5’-Cytosolic nucleotidase IIIB (cN-IIIB) is one of the most recently discovered 5’-nucleotidases and has several unique structural and functional features. However, one of the most preferred cN-IIIB substrates is m7GMP, for which the activity of dephosphorylation is characterized by one order of magnitude lower KM constant compared to the other preferred substrates, whereas kcat/KM is comparable. The crystal structure of cN-IIIB consists of two distinct domains: the globular core domain (residues 1–51, 132–182, and 215–300) and the smaller CAP domain (52–131 and 183–214). The core domain is a haloacid dehalogenase domain (HAD).

To date, these are the first coordinates obtained for human cytosolic nucleotidase IIIB. The second domain mainly consists of a bundle of helices that are responsible for recognizing the ligand. The C-terminal part of the protein (residues 291–300) and one of a loop connecting domains (residues 211–220) were not defined in the electron density map, and thus are most likely disordered. In all three crystal structures, the magnesium ion was octahedrally coordinated by the carboxyl side chains of catalytic moieties of Asp 41 and Asp 230 and the backbone carbonyl of Asp 43 and by three water molecules. The differences between solved structures: the holoenzyme of cN-IIIB • Mg2+, and the enzyme in complex with inhibitors: 5d or 5d’, concern mainly two helices of the CAP domain, which move slightly down and left towards HAD domain by about 3 Å. Ligand-binding triggers substantial changes of Tyr60 and Trp105 sidechain conformations to form a system of aromatic rings that stabilize the complex. Crystals appeared in a few days at 4 °C after mixing protein with 0.1 M MES (pH 6.2) and 22–28% PEG 3350.

> RSMAEEVSTLMKATVLMRQPGRVQEIVGALRKGGGDRLQVISDFDMTLSRFAYNGKRCPSSYNILDNSKIISEECRKELTALLHHYYPIEIDPHRTVKEKLPHMVEWWTKAHNLLCQQKIQKFQIAQVVRESNAMLREGYKTFFNTLYHNNIPLFIFSAGIGDILEEIIRQMKVFHPNIHIVSNYMDFNEDGFLQGFKGQLIHTYNKNSSACENSGYFQQLEGKTNVILLGDSIGDLTMADGVPGVQNILKIGFLNDKVEERRERYMDSYDIVLEKDETLDVVNGLLQHILCQGVQLEMQGP>MSAIKDSRNINFNTKHLRKGDPLPPFNGKLRVYNMRYCPYAQRTILALNAKQIDYEVVNIDLIDKPEWLTTKSAFAKVPAIEIAEDVTIYESLVTVEYLDEVYPKRPLLPQDPLKKALDKIIVEASAPIQSLFIKILKFSDTVNEEHVAAYHKALDFIQEQLKNRGTVFLDGSEPGYADYMIWPWFERLRAFAHDERVRLEPSKYSLLLEYIDNMLKDSAVSQYLIPLEILAKFHEAYTKKERPNYELLNECLKSF[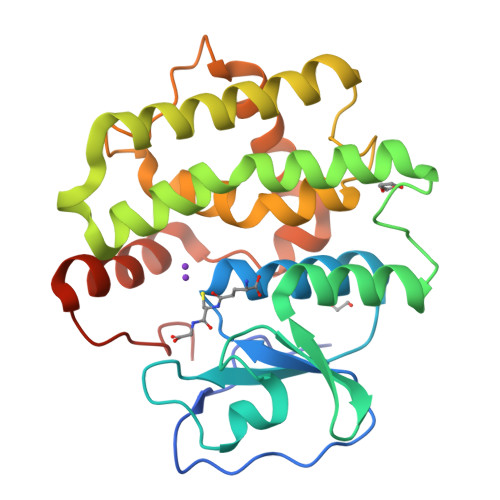4x]Acetobacter aceti strain 1023 and other acetic acid bacteria use succinyl-CoA:acetate CoA-transferase (AarC) in a variant citric acid cycle that is required for a robust acetic acid resistance (aar) phenotype. Strong selection for key roles in acetic acid resistance and central metabolism appear to have optimized the structural and functional properties of AarC, making it an excellent representative of the class I CoA-transferase superfamily. Class I acyl-CoA:carboxylate CoA-transferases produce reactive acylglutamyl anhydride intermediates that acylate CoA, forming either an acyl-CoA product and a free enzyme or a protein glutamyl-CoA thioester and a carboxylate product. A closed active site enables AarC to engage, immobilize, and desolvate acyl-CoA substrates and to stabilize covalent adducts of Glu294.

Acetic acid or acetate (collectively “acetate”) has been observed in several AarC structures without being provided in the crystallization solution. The final model contained three acetate binding sites in each subunit, related by the pseudo-twofold axis. Acetate (ACT 606A and 603B) accepts hydrogen bonds from the side chains of Ser71, Thr94, and Arg228. This is the only acetate binding site not located at the rather polar interface between subunits. The second acetate binding site overlaps a chloride binding site (CL 515) observed in earlier structures and is located on the flanks of the dimer. Acetate (ACT 605A and ACT 605B) accepts hydrogen bonds from the side chains of Asn112, Arg120, and Asn125 of the same subunit and the backbone of Gly443′ (the prime denotes a residue from the partner subunit). The third acetate binding site overlaps the other chloride binding site (CL 516) observed in earlier structures and is located near the pseudo-twofold axis on the flat “top” of the dimer. Acetate (ACT 607A and 601B) accepts hydrogen bonds from the side chains of Arg354 (bidentate) and Arg354′ (monodentate) and the backbone NH of Val196′. Protein atoms in the interfacial acetate and chloride binding sites are nearly superimposable, indicating that the acetate displaces chloride ions supplied by the buffers used to isolate and crystallize recombinant AarC(H6). As anticipated, each subunit in the AarC•acetate complex possesses active site parameters typical of other open conformations.

>MTERIRNVALRSKVCPAETASELIKHGDVVGTSGFTGAGYPKEVPKALAQRMEAAHDRGEKYQISLITGASTGPQLDGELAKANGVYFRSPFNTDATMRNRINAGETEYFDNHLGQVAGRAVQGNYGKFNIALVEATAITEDGGIVPTSSVGNSQTFLNLAEKVIIEVNEWQNPMLEGIHDIWDGNVSGVPTRDIVPIVRADQRVGGPVLRVNPDKIAAIVRTNDRDRNAPFAAPDETAKAIAGYLLDFFGHEVKQNRLPPSLLPLQSGVGNVANAVLEGLKEGPFENLVGYSEVIQDGMLAMLDSGRMRIASASSFSLSPEAAEEINNRMDFFRSKIILRQQDVSNSPGIIRRLGCIAMNGMIEADIYGNVNSTRVMGSKMMNGIGGSGDFARSSYLSIFLSPSTAKGGKISAIVPMAAHVDHIMQDAQIFVTEQGLADLRGLSPVQRAREIISKCAHPDYRPMLQDYFDRALKNSFGKHTPHLLTEALSWHQRFIDTGTMLPSSLEHHHHHH[2x]Galectins are a family of proteins with some specificity for β-galactoside binding at their carbohydrate-recognition domain (CRD). Tandem-repeat-type galectins, like Gal-8, contain two distinct CRDs that are covalently connected via a peptide linker. In the present study, we used different conditions to crystallize the Gal-8 N-terminal CRD with its linker, and five structures could be solved. The N-terminal CRD prefers sulfated and sialylated glycans, whereas the C-terminal CRD prefers blood group A/B. In particular, the N-terminal CRD strongly binds to sulfated and sialylated glycans.

Our five structures were solved from crystals grown under two different conditions: (1) 20% (w/v) PEG2000 MME and (2) 0.1 M Tris pH 8.5, 0.01 M NiCl2, 20% (w/v) PEG2000 MME. Structures 4 and 5 were solved from the second condition and cryoprotectants for these two structures were glycerol and ethylglycol, respectively. Unfortunately, the structure of the linker could not be defined, because following crystal structure refinement, no electron density for the linker was observed (from Ser154 to end), indicating that the linker is highly flexible. In structures 4 and 5, the electron density of residues from Ser154 to the C-terminus was not visible, suggesting greater flexibility from this segment. In structures 1–3, the N terminal tail (Gln9 to Ile12) forms a rigid loop, whereas in structures 4 and 5, the N terminal tail (Gln9 to Ile12) forms a small β-strand F0. In structures 4 and 5, Ni2+ formed a complex with Asp25 and His38, His147 from another Gal-8N molecule, along with three water molecules. Asp25 is close to β-strand S1, and coordination between Asp25 and Ni2+ may impact on S1. Therefore, S1 may induce Gln9 to Ile12 to form a β-strand from Ile12 to Phe19 via van der Waals forces. If the N-terminal tail interacts with the linker, then Gln9 to Ile12 forms a rigid loop and part of the linker (here is from Ser154 to Gln158) is stabilized. In contrast, if the N-terminal tail cannot interact with the linker for some reason (e.g., due to the Ni2+ ion mentioned above), then Gln9 to Ile12 forms a β-strand with the linker having high flexibility. In our P43212 structure, glycerol also could not replace lactose.

> GSHMMLSLNNLQNIIYNPVIPFVGTIPDQLDPGTLIVIRGHVPSDADRFQVDLQNGSSMKPRADVAFHFNPRFKRAGCIVCNTLINEKWGREEITYDTPFKREKSFEIVIMVLKDKFQVAVNGKHTLLYGHRIGPEKIDTLGIYGKVNIHSIGFSFSSDLQSTQASSLELTEISRENVPKSGTPQLRLP> SLEARAALNQALEMKRQGKREKAQKLFMHALKMDPDFVDALTEFGIFSEEDKDIIQADYLYTRALTISPYHEKALVNRDRTLPLVEEIDQRYFSIIDSKVKKVMSIPKGNSALRRVMEETYYHHIYHTVAIEGNTLTLSEIRHILETRYAVPGASLEEQNEVIGMHAAMKYINTTLVSRIGSVTISDVLEIHRRVLGYVDPVEAGRFRTTQVLVGHHIPPHPQDVEKQMQEFVQWLNSEEAMNLHPVEFAALAHYKLVYIHPFIDGNGRTSRLLMNLI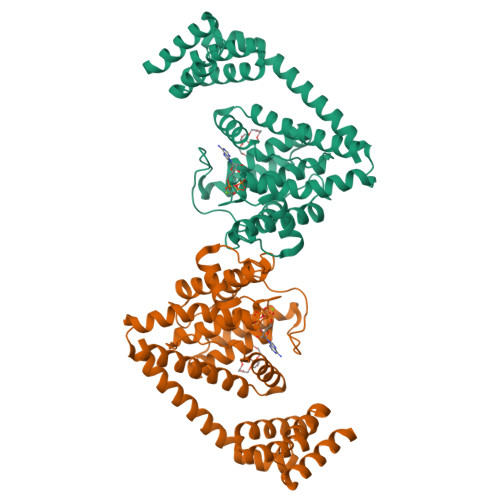LMQAGYPPITIRKEQRSDYYHVLEAANEGDVRPFIRFIAKCTETTLDTLLFATTEYSVALPEAQP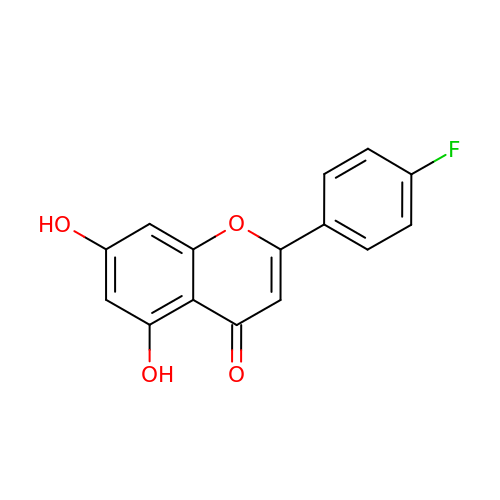2-(4-fluorophenyl)-5,7-bis(oxidanyl)chromen-4-one | C15 H9 F O4 | XSYORHATJHJUAA-UHFFFAOYSA-N>[2x]GSNKLHLRVVTLIEHPFVFTREVDDEGLCPAGQLCL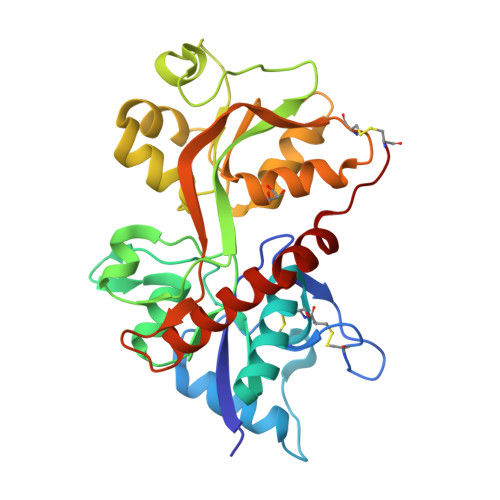DPMTNDSSMLDRLFSSLHSSNDTVPIKFKKCCYGYCIDLLEQLAEDMNFDFDLYIVGDGKYGAWKNGHWTGLVGDLLSGTANMAVTSFSINTARSQVIDFTSPFFSTSLGILVRTRGTELSGIHDPKLHHPSQGFRFGTVRESSAEDYVRQSFPEMHEYMRRYNVPATPDGVQYLKNDPEKLDAFIMDKALLDYEVSIDADCKLLTVGKPFAIEGYGIGLPPNSPLTSNISELISQYKSHGFMDVLHDKWYKVVPCGK4-({1-[3-(3-amino-3-oxopropyl)-5-chlorophenyl]-3-methyl-1H-pyrazolo[4,3-c]pyridin-6-yl}amino)-3-methoxy-N-(1-methylpiperidin-4-yl)benzamide | C30 H34 Cl N7 O3 | 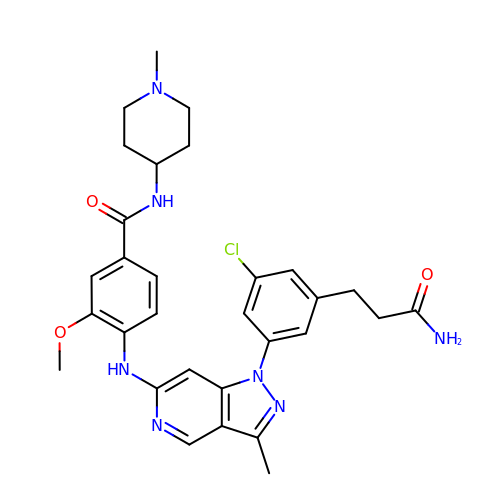NRECIWMNKXRLNI-UHFFFAOYSA-N> MGFLELDTNLPANRVPAGLEKRLCAA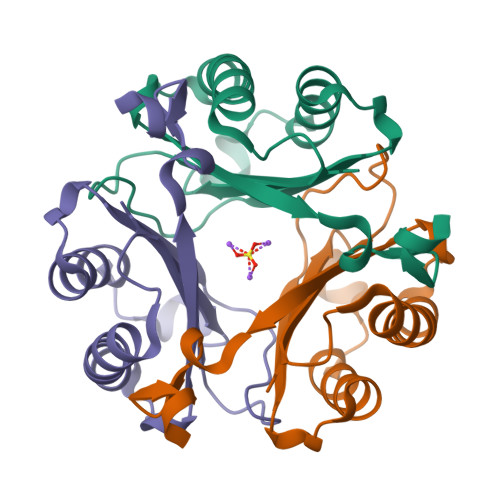AASILGKPADRVNVTVRPGLAMALSGSTEPCAQLSISSIGVVGTAEDNRSHSAHFFEFLTKELALGQDRILIRFFPLESWQIGKIGTVMTFL3-ACETYLPYRIDINE ADENINE DINUCLEOTIDE PHOSPHATE | C22 H29 N6 O17 P3 | 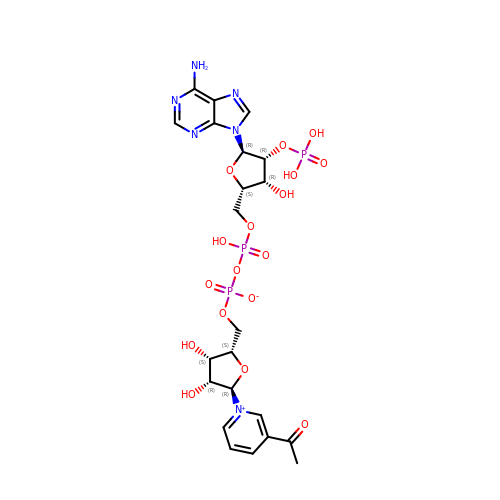CWZSJEPJRFQEBR-SIEFPTHMSA-N> HPICEVSKVASHLEVNCDKRQLTALPPDLPKDTTILHLSENLLYTFSLATLMPYTRLTQLNLDRCELTKLQVDGTLPVLGTLDLSHNQLQSLPLLGQTLPALTVLDVSFNRLTSLPLGALRGLGELQELYLKGNELKTLPP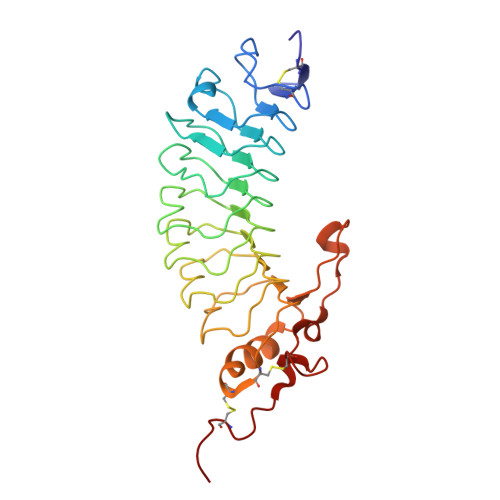GLLTPTPKLEKLSLANNQLTELPAGLLNGLENLDTLLLQENSLYTIPKGFFGSHLLPFAFLHGNPWLCNCEILYFRRWLQDNAENVYVWKQGVDVKAMTSNVASVQCDNSDKFPVYKYPGKGCPLVPR>[2x]MGHHHHHHGGGENLYFQGSMQPDMSLNVIKMKSSDFLESAELDSGGFGKVSLAFHRTQGLMIMKTVYKGPNCIEHNEALLEEAKMMNRLRHSRVVKLLGVIIEEGKYSLVMEYMEKGNLMHVLKAEMSTPLSVKGRIILEIIEGMAYLHGKGVIHKDLKPENILVDNDFHIKIADLGLASFKMWSKLNNEEHNELREVDGTAKKNGGTLYYMAPEHLNDVNAKPTEKSDVYSFAVVLWAIFANKEPYENAIAEQQLIMAIKSGNRPDVDDITEYCPREIISLMKLCWEANPEARPTFPGIEEKFRPFYLSQLE

The necrosome comprises receptor-interacting serine/threonine-protein kinase 1 (RIPK1), RIPK3, and mixed lineage kinase domain-like protein (MLKL). , Active RIPK1 phosphorylates and activates RIPK3, which in turn phosphorylates MLKL. Formation of the necrosome involves RIPK1 autophosphorylation at multiple sites, followed by phosphorylation of RIPK3, and finally MLKL phosphorylation, which initiates pore formation and necroptosis. Necroptosis is a form of programmed cell death that, when dysregulated, is associated with cancer and inflammatory and neurodegenerative diseases. Here, we describe a multifaceted array of molecular, cellular, structural, and chemical biology approaches to characterize the 7PQ inhibitor series and identify RIPK1 as their target.

RIPK1 was purified and crystallized in the presence of Nec-1s followed by soaking with AZ’902 or AZ’320. Nec-1s is an allosteric inhibitor of RIPK1, and binding was observed at a hydrophobic pocket behind the ATP binding site, as previously described. In contrast, AZ’902 and AZ’320 both bound RIPK1 at identical sites around the hinge region, with the 7PQ motif interacting directly with RIPK1. A hydrogen bond interaction was identified between the 7PQ nitrogen and the backbone nitrogen of RIPK1 Met95, supporting the critical position of the nitrogen observed in the SAR studies and explaining the inactivity of compounds in which this nitrogen is varied. The compounds partially overlap with the predicted ATP binding site and thus likely act as Type I kinase inhibitors; as per literature, most inhibitors for RIPK1 are Type II or III. The RHS of the molecules is exposed to the solvent and does not form notable interactions with RIPK1, consistent with the observation that a range of motifs are tolerated in the para-position of the 7-phenyl ring. Furthermore, incubation with AZ’902 led to significant changes in HDX exchange at the hinge region around Met95 (residues 94–100), with the same trend observed for AZ’320. Given the precedence for inhibition of RIPK1 to prevent necroptosis, the possibility of direct RIPK1 inhibition was tested in a biochemical ADP-Glo kinase assay using the recombinant RIPK1 kinase domain. Both AZ’902 and Nec-1 inhibited RIPK1 kinase activity with comparable IC50s, confirming the 7PQ series as inhibitors of RIPK1. Nec-1s and AZ’902 acted synergistically specifically in the range of 0.06–0.25 μM Nec-1s and 0.78–3.13 μM AZ’902, using the HSA model in the Combenefit analysis package. Key structural motifs adjacent to the Nec-1s allosteric site, such as the DFG loop and C-α helix, are in the same inactive conformation observed when Nec-1s is bound to RIPK1 alone, suggesting that the mechanism of Nec-1s binding is unaffected by the 7PQ series.(2S,3R,4E)-3-hydroxy-2-(octanoylamino)octadec-4-en-1-yl 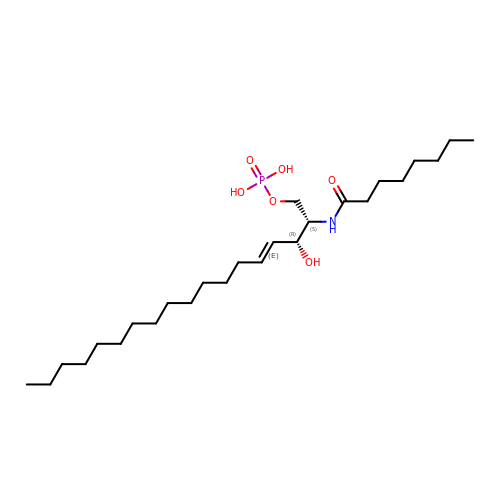dihydrogen phosphate | C26 H52 N O6 P | VSSNYUXSRXINIP-WRBRXSDHSA-N>MSDAKVFGKCEFAELLKRDYYLSNDDIKNWVCIAEFESSFNTAAINRNRNRSTDYGIFQINNKYWCGSDYGKNVCKIPCSDLMSDDITEALRCAETIRRDTERFRGRGKGYSAWVAYNSKCKNRDLDQYMAECWSHGSNSV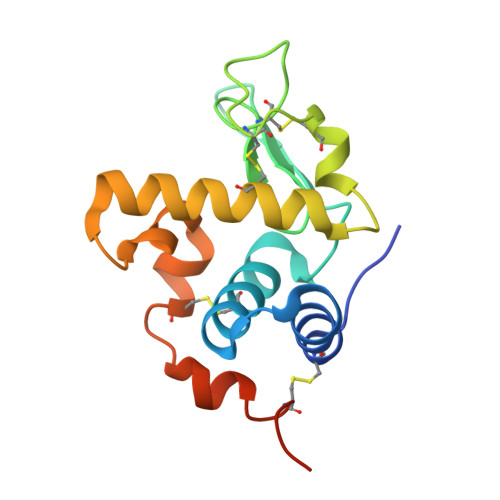FPF[2x]> M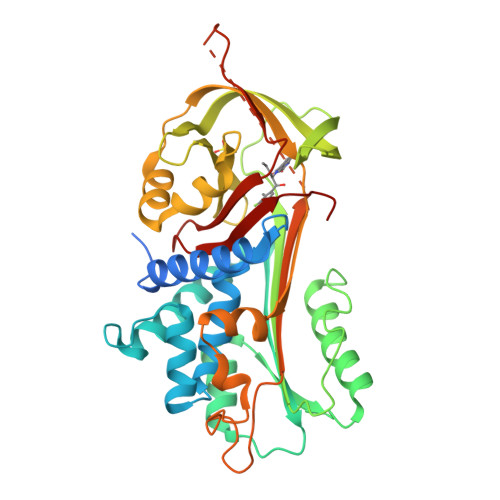RGSHHHHHHTDPQGDAAQKTDTSHHDQDHPTFNKITPNLAEFAFSLYRQLAHQSNSTNIFFSPVSIATAFAMLSLGTKADTHDEILEGLNFNLTEIPEAQIHEGFQELLRTLNQPDSQLQLTTGNGLFLSEGLKLVDKFLEDVKKLYHSEAFTVNFGDTEEAKKQINDYVEKGTQGKIVDLVKELDRDTVFALVNYIFFKGKWERPFEVKDTEEEDFHVDQVTTVKVPMMKRLGMFNIQHSKKLSSWVLLMKYLGNATAIFFLPDEGKLQHLENELTHDIITKFLENEDRRSASLHLPKLSITGTYDLKSVLGQLGITKVFSNGADLSGVTEEAPLKLSKAVHKAVLTIDEKGTEAAGAMFLEAIPMSIPPEVKFNKPFVFLMIEQNTKSPLFMGKVVNPTQK>MANKQDLIAKVAEATELTKKDSAAAVDAVFSAVSSYLAKGEKVQLIGFGNFEVRERAARKGRN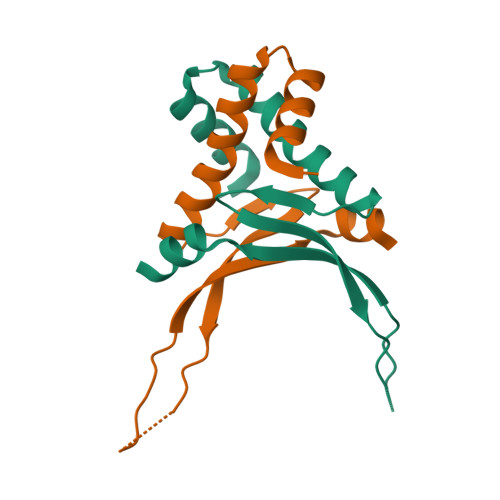PQTGEEIKIKASKVPAFKAGKALKDAVKHHHHHHHH[2x]>[2x]GMNDLKRLPYEPVKGLLPRPAVGTSERVITLPEPDRTSGMPLMGTLWLRKSTREFDQQPLPLKQLSELLWAAAG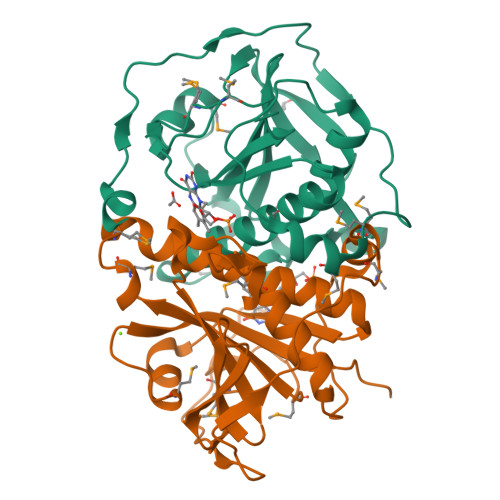VNRSLGGGRTAPSPYGETVIDVYVALPAGLYRYDPVHHCLELKRAADLRSMTGYQDFVGMAPLDLVFVANHGRMQEMPPKLRETFSAAAAGAMAENAYLYCASAGLGAVVRGWLNRRQLAEHMSLNEDEEPILSQTIGRAASHVTTTQA>MSNEDLFICIDHVAYACPDADEASKYYQETFGWHELHREENPEQGVVEIMMAPAAKLTEHMTQVQVMAPLNDESTVAKWLAKHN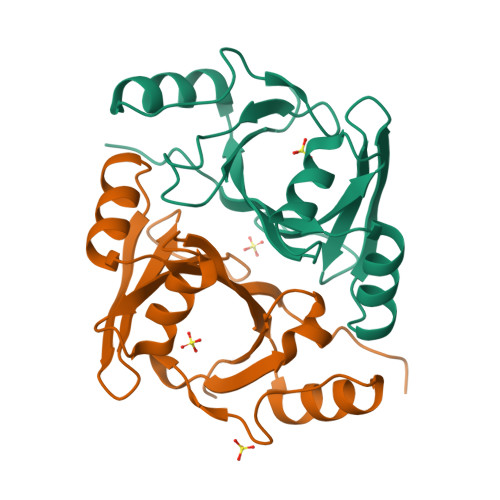GRAGLHHMAWRVDDIDAVSATLRERGVQLLYDEPKLGTGGNRINFMHPKSGKGVLIELTQYPKN[6x]>MGHHHHHHMTPKRALISLTSYHGPFYKDGAKTGVFVVEILRSFDTFEKHGFEVDFVSETGGFGWDEHYLPKSFIGGEDKMNFETKNSAFNKALARIKTANEVNASDYKVFFASAGHGALFDYPKAKNLQDIASKIYANGGVIAAICHGPLLFDGLIDIKTTRPLIEGKA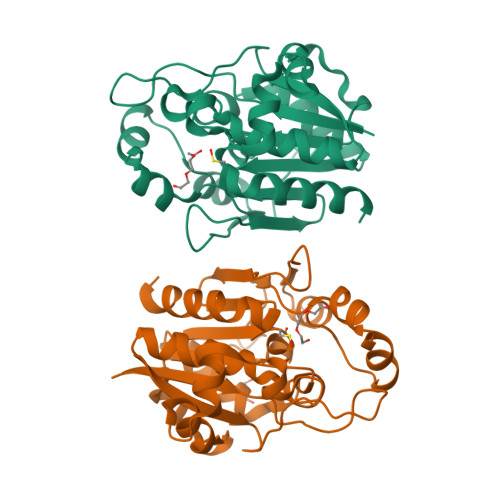ITGFPLEGEIALGVDDILRSRKLTTVERVANKNGAKYLAPIHPWDDYSITDGKLVTGVNANSSYSTTIRAINALYS[2x]> MEPLKVEKFATANRGNGLRAVTPLRPGELLFRSDPLAYTVCKGSRGVVCDRCLLGKEKLMRCSQCRVAKYCSAKCQKKAWPDHKRECKCLKSCKPRYPPDSVRLLGRVVFKLMDGAPSESEKLYSFYDLES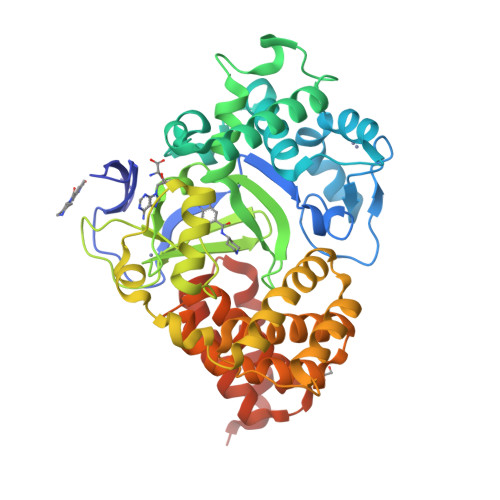NINKLTEDKKEGLRQLVMTFQHFMREEIQDASQLPPAFDLFEAFAKVICNSFTICNAEMQEVGVGLYPSISLLNHSCDPNCSIVFNGPHLLLRAVRDIEVGEELTICYLDMLMTSEERRKQLRDQYCFECDCFRCQTQDKDADMLTGDEQVWKEVQESLKKIEELKAHWKWEQVLAMCQAIISSNSERLPDINIYQLKVLDCAMDACINLGLLEEALFYGTRTMEPYRIFFPGSHPVRGVQVMKVGKLQLHQGMFPQAMKNLRLAFDIMRVTHGREHSLIEDLILLLEECDANIRASFULL phenazin-1-ol | C12 H8 N2 O | 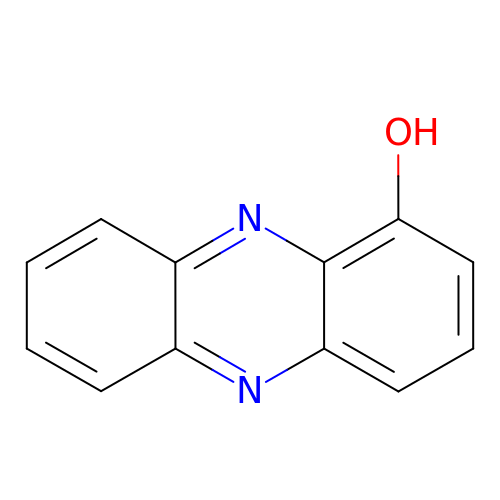SVRNCBGWUMMBQB-UHFFFAOYSA-N> MSEVITITKRNGAFQNSSNLSYNNTGISDDENDEEDIYMH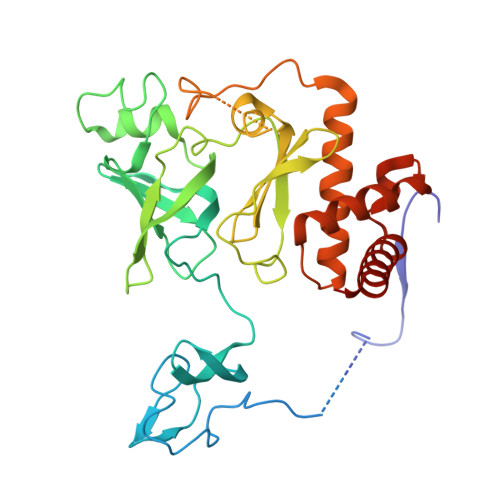DVNSASKSESDSQIVTPGELVTDDPIWMRGHGTYFLDNMTYSSVAGTVSRVNRLLSVIPLKGRYAPETGDHVVGRIAEVGNKRWKVDIGGKQHAVLMLGSVNLPGGILRRKSESDELQMRSFLKEGDLLNAEVQSLFQDGSASLHTRSLKYGKLRNGMFCQVPSSLIVRAKNHTHNLPGNITVVLGVNGYIWLRKTSQMDLARDTPSANNSSSIKSTGPTGAVSLNPSITRLEEESSWQIYSDENDPSISNNIRQAICRYANVIKALAFCEIGITQQRIVSAYEASMVYSNVGELIEKNVMESIGSDILTAEKMRGNGN(3R,4S)-4-[(4-fluorobenzoyl)amino]-6-[4-(oxetan-3-yl)piperazin-1-yl]-3,4-dihydro-2H-chromen-3-yl methylcarbamate 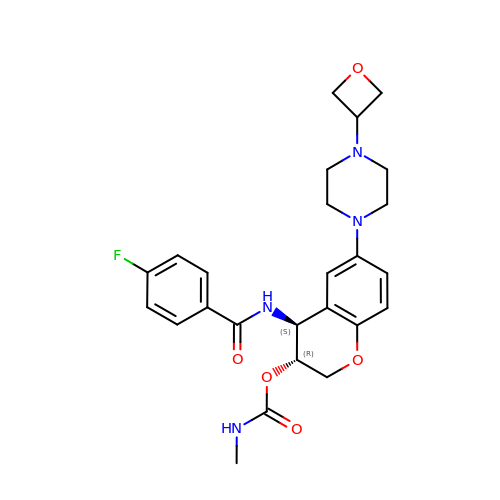| C25 H29 F N4 O5 | NDEBZCZEAVMSQF-GOTSBHOMSA-N> MDIAIVDADNPADAIQQVKDLRKYGAKLIAYKSKSSEELKLALKAGADIAIVDADNPADAIQQVKD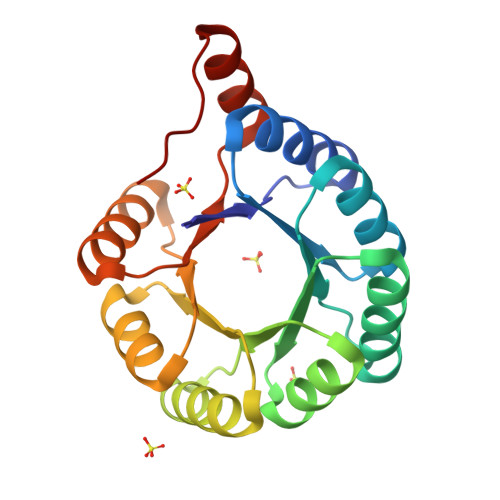LRKYGAKLIAYKSKSSEELKLALKAGADIAIVDADNPADAIQQVKDLRKYGAKLIAYKSKSSEELKLALKAGADIAIVDADNPADAIQQVKDLRKYGAKLIAYKSKSSEELKLALKAGHHHHHH One of the key proteins in long-term synaptic plasticity and memory is the activity-regulated cytoskeleton-associated protein (Arc). Drosophila has two isoforms of Arc, dArc1 and dArc2, with low sequence similarity to mammalian Arc, but lacking a large N-terminal domain. Both dArc isoforms are related to the Ty3/gypsy retrotransposon capsid, consisting of N- and C-terminal lobes. As opposed to the corresponding mammalian Arc lobe domains, which are monomeric, the dArc lobes were all oligomeric in solution, indicating a strong propensity for homophilic interactions.

Each monomer consists of five helices in an orthogonal bundle fold, and the structures are highly similar to each other. The dimer interface is in both cases formed by α1 and α3 from each monomer, and the total buried surface area at the interface is ~1400 Å2. Both interfaces contain four hydrogen bonds and four salt bridges. The interface is conserved, displaying only three conservative replacements between the isoforms (A125/L170/F172 in dArc1 to S112/F157/Y159 in dArc2). (D) A comparison of the dArc-CL crystal structures with the same domains in dArc capsids. Both the dArc1 and dArc2 C-lobes closely resemble their counterparts in the capsids, with an all-atom RMSD of 1.75 Å2 and 1.13 Å2, respectively. The dimer interface in dArc-CL, which corresponds to that in retroviral CA-CTD, contains mainly hydrophobic interactions; half of these hydrophobic residues are polar in the rat Arc-CL, and the first helix of the dArc-CL, a major part of the dimer interface, is tilted away in mArc, possibly explaining the monomeric state of mArc-CL in solution. The most conserved residue (Gln124 in dArc2) is structurally important, forming hydrogen bonds and contacts with many neighbours, including the conserved residues Phe133 and Met162. Kratky plots also indicate that dArc1-CL is more flexible than dArc2-CL.

>[4x]SGSGKPSYQIYMEIFETKQSYDEVIDSFICKQRALLAKLPEGRHDEETELDFIYGLMQPKYRESIPRHEVKTFRELLDRGRTVERTRH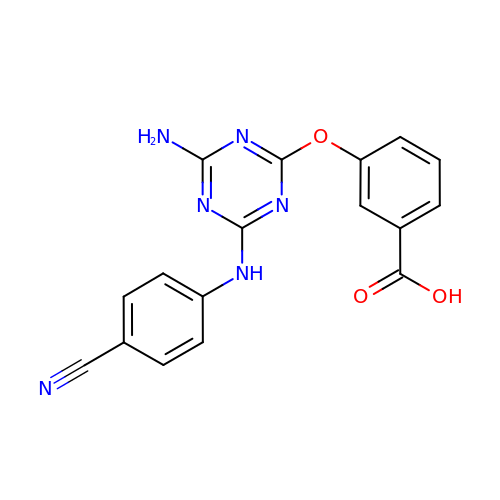3-({4-amino-6-[(4-cyanophenyl)amino]-1,3,5-triazin-2-yl}oxy)benzoic acid | C17 H12 N6 O3 | WKFGNLUJVJDVRJ-UHFFFAOYSA-N>GPSLGYCCGRKLEFSPQTLCCYGKQLCTIPRDATYYSYQNRYHFCEKCFNEIQGESVSLGDDPSQPQTTINKEQFSKRKNDTLDPELFVECTECGRKMHQICVLHHEIIWPAGFVCDGCLKKSARTRKENKFSAKRLPSTRLGTFLENRVNDFLRRQNHPESGEVTVRVVHASDKTVEVKPGMKARFVDSGEMAESFPYRTKALFAFEEIDGVDLCFFGMHVQEYGSDCPPPNQRRVYISYLDSVHFFRPKCLRTAVYHEILIGYLEYVKKLGYTTGHIWACPPSEGDDYIFHCHPPDQKIPKPKRL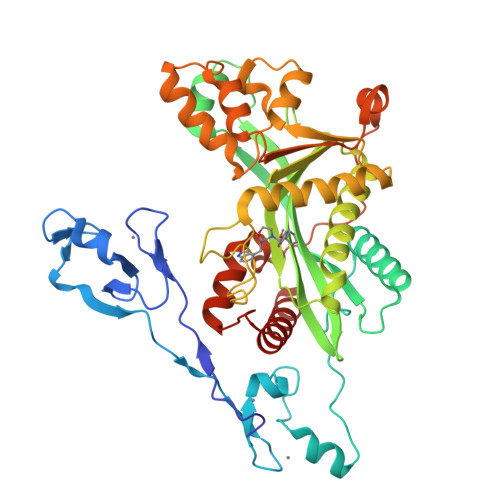QEWFKKMLDKAVSERIVHDYKDIFKQATEDRLTSAKELPYFEGDFWPNVLEESIKESGGSGSQKLYATMEKHKEVFFVIRLIAGPAANSLPPIVDPDPLIPCDLMDGRDAFLTLARDKHLEFSSLRRAQWSTMCMLVELHTQSQDRF[2x]>[2x]MSPLSGSLAPLNMKGLVKFQDVSFAYPNHPNVQVLQGLTFTLYPGKVTALVGPNGSGKSTVAALLQNLYQPTGGKVLLDGEPLVQYDHHYLHTQVAAVGQEPLLFGRSFRENIAYGLTRTPTMEEITAVAMESGAHDFISGFPQGYDTEVGETGNQLSGGQRQAVALA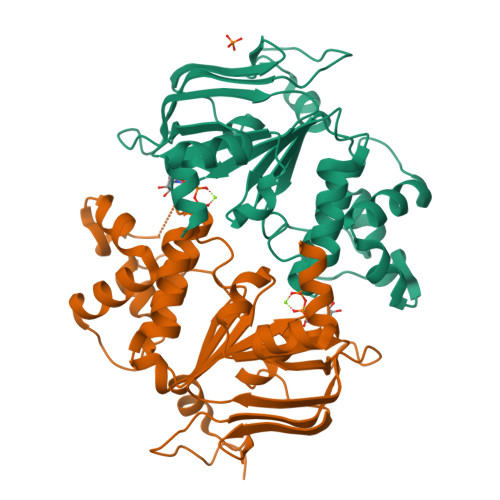RALIRKPRLLILDNATSALDAGNQLRVQRLLYESPEWASRTVLLITQQLSLAERAHHILFLKEGSVCEQGTHLQLMERGGCYRSMVEALAAPSDAAAHHHHHH> SMPKTISVRVTTMDAELEFAIQPNTTGKQLFDQVVKTIGLREVWFFGLQYQDTKGFSTWLKLNKKVTAQDVRKESPLLFKFRAKFYPEDVSEELIQDITQRLFFLQVKEGILNDDIYCPPETAVLLASYAVQSKYGDFNKEVHKSGYLAGDKLLPQRVLEQHKLNKDQWEERIQVWHEEHRGMLREDAVLEYLKIAQDLEMYGVNY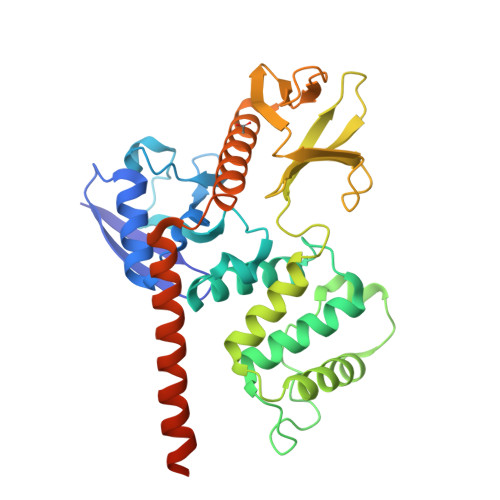FSIKNKKGSELWLGVDALGLNIYEQNDRLTPKIGFPWSEIRNISFNDKKFVIKPIDKKAPDFVFYAPRLRINKRILALCMGNHELYMRRRKPDTIEVQQMKAQAREEKHQKQMERAMLENEKKKREMAEKEKEKIEREKEE>[10x]MTQSLHYSSPRETLTDTIMMAKIR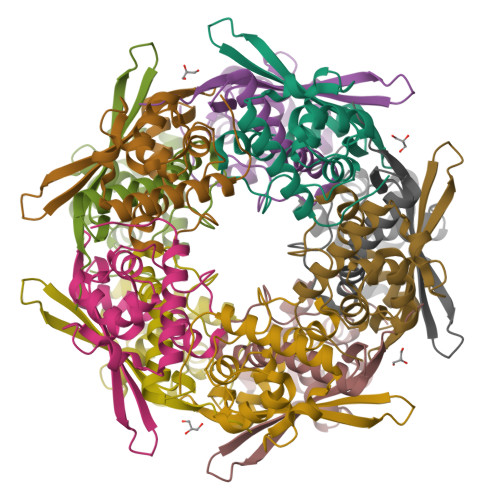KNLTFEAINQGTGLSLAFVTAALLGQHPLPEQAARVVAEKLDLDEDAIRLLQTIPLRGSIPGGVPTDPTIYRFYEMVQIYGSTLKALVHEQFGDGIISAINFKLDIKKVPDPDGGERAVITLDGKYLPTKPF> GHMSSTPSNQNIIPIIKKESIVSLFEKGIRQDGRKLTDYRPLSITLDYAKKADGSALVKLGTTMVLAGTKLEIDKPYEDTPNQGNLIVNVELLPLAYETFEPGPPD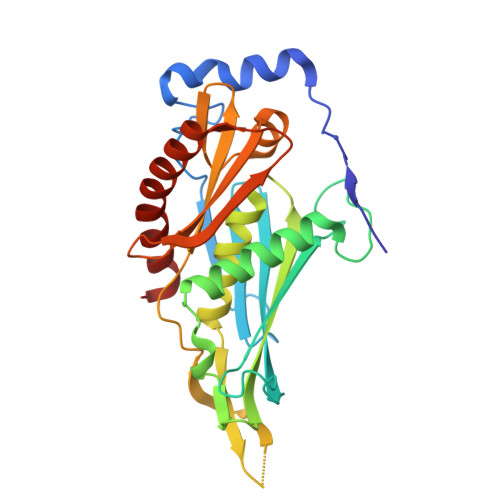ENAIELARVVDRSLRDSKALDLTKLVIEPGKSVWTVWLDVYVLDYGGNVLDACTLASVAALYNTKVYKVEQHSNGISVNKNEVVGKLPLNYPVVTISVAKVDKYLVVDPDLDEESIMDAKISFSYTPDLKIVGIQKSGKGSMSLQDIDQAENTARSTAVKLLEELKKHLGI4-nitrophenyl 1-thio-beta-D-glucopyranoside | C12 H15 N O7 S | 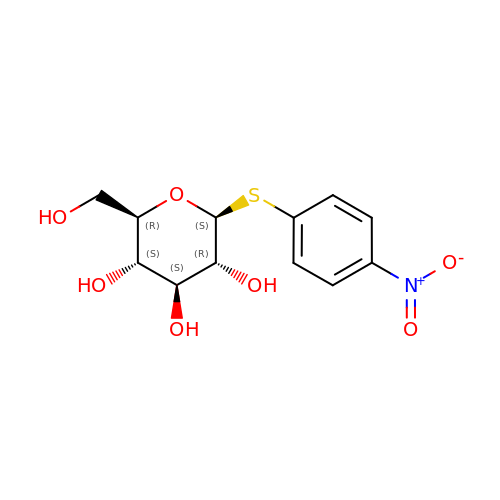IXFOBQXJWRLXMD-ZIQFBCGOSA-N>[2x]SVRPVIGSVAPESLAAQAGLEAGQELLAVDGEPVTGWNGVNLQLVRRLGESGT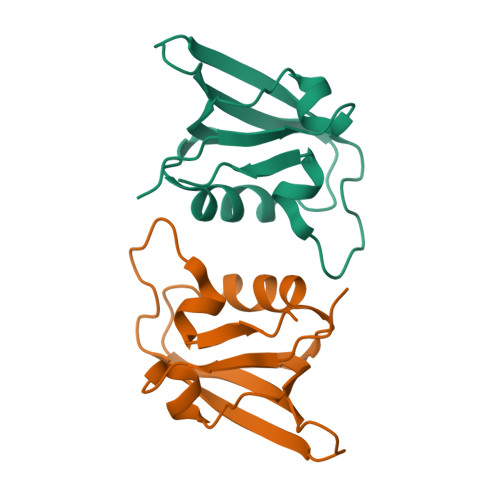LEVRVQEKGSNVDSTHQVRLDGWLKGEDNPDPIASLGIRPWRP2-amino-7-(1-methylethyl)-5-oxo-5H-chromeno[2,3-b]pyridine-3-carboxylic acid | C16 H14 N2 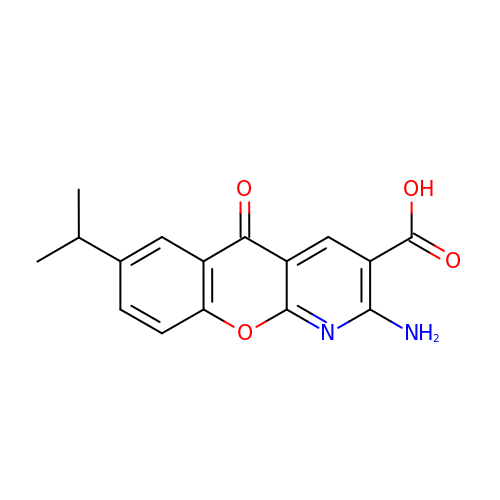O4 | SGRYPYWGNKJSDL-UHFFFAOYSA-N> ARTVVLITGCSSGIGLHLAVRLASDPSQSFKVYATLRDLKTQGRLWEAARALACPPGSLETLQLDVRDSKSVAAARERVTEGRVDVLVCNAGLGLLGPLEALGEDAVASVLDVNVVGTVRMLQAFLPDMKRRGSGRVLVTGSVGGLMGLPFNDVYCASKFALEGLCESLAVLLLPFGVHLSLIECGPVHTAFMEKVLGSPEEVLDRTDIHT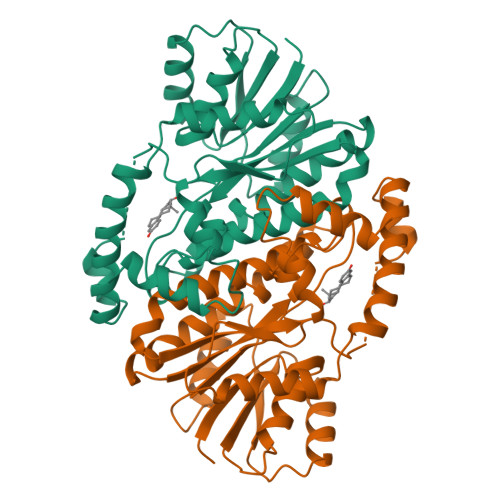FHRFYQYLAQSKQVFREAAQNPEEVAEVFLTALRAPKPTLRYFTTERFLPLLRMRLDDPSGSNYVTAMHREVFGDVPAKAEAGAEAGGGRGPGAEDEAGRSAVGDPELGDPPAAPQ>[5x]NAMIIRPEQHWFLRLFDWHGSVLSKIIFRLLLNVLMSIIAIISYQWYEQLGIHLTVAPFSLLGIAIAIFLGFRNSASYSRFVEARNLWGTVLIAERTLVRQLRNILPAEHDAHRRIVSYLVAFSWSLKHQLRKTDPTADLRRLLPEERVTEILASSMPTNRILLLAGNEIGQLREAGKLSDITYGLMDNKLDELAHVLGGCERLATTPVPFAYTLILQRTVYLFCTLLPFALVGDLHYMTPFVSVFISYTFLSADSLAEELEDPFGTAANDLPLNAMCNTIERNLLDMTGQHPLPE

Human bestrophin1 (hBest1) is a Ca2+-activated Cl− channel essential for Cl− transport in retinal pigment epithelium (RPE). Although the structure of hBest1 is still unsolved, two Best1 homolog structures, one from bacteria Klebsiella pneumoniae (KpBest) and the other from chicken (cBest1), have been previously reported. Overall, the channel is a pentameric assembly with a single ion-conducting pathway, which varies in diameter along its length and is constrained at two narrow points: a “neck” contributed by three residues (I62/I66/F70 in KpBest and I76/F80/F84 in hBest1/cBest1) on a transmembrane helix, and an “aperture” formed by a single residue (I180 in KpBest1, I205 in hBest1, and V205 in cBest1) on a cytosolic helix. Here, by electrophysiological and structural analyses, we show that the neck and aperture in hBest1 are both indispensable Ca2+-dependent gates, and their dysregulated opening by rationally designed or patient-derived mutations causes Ca2+-independent leak and elevates Ca2+-dependent channel activity.

By sharp contrast, cells expressing hBest1 W287A conducted tiny current just like untransfected cells, suggesting that, to the opposite of W287F, W287A is a loss-of-function mutation. Therefore, W287 is an extremely sensitive “switch” of the neck. To understand the structural bases of these mutants, we solved the structures of KpBest Y211A, W252A, and W252F at 2.6, 2.5, and 3.1 Å (equivalent to hBest1 Y236A, W287A, and W287F), respectively. Consistent with the functional results, no structural change was found at the aperture. Although the structure at the neck region was surprisingly unaltered, possibly due to the molecular packing effect in the crystal or the presence of Zn2+ in the crystallization solution which might stabilize the channel in a closed state, all three KpBest mutants displayed conformational changes on P208, Y211, and W252 (equivalent to P233, Y236, and W287 in hBest1, respectively), reaffirming the mutual influence between these three residues. Taken together, we concluded that hBest1 P233, Y236, and W287 are critical residues involved in channel gating at the neck.> YTPVEEKENGRMIVIVPKKYEEDIEDFVDWKNQRGLRTEVKVAEDIASPVTANAIQQFVKQEYEKEGNDLTYVLLVGDHKDIPAKITPGIKSDQVYGQIVGNDHYNEVFIGRFSCESKEDLKTQIDRTIHYERNITTEDKWLGQALCIASAEGGPSADNGESDIQHENIIANLLTQYGYTKIIKCYDPGVTPKNIIDAFNGGISLANYTGHGSETAWGTSHFGTTHVKQLTNSNQLPFIFDVACVNGDFLYNVPCFAEALMRAQKDGKPTGTVAIIASTINQSWASPMRGQDEMNEILCEKHPNNIKRTFGGVTMNGMFAMVEKYKKDGEKMLDTWTVFGDPSLLVRTLVPTKMQVTAPANISASAQTFEVACDYNGAIATLSDDGDMVGTAIVKDGKAIIKLNESIADETNLTLTVVGYNKVTV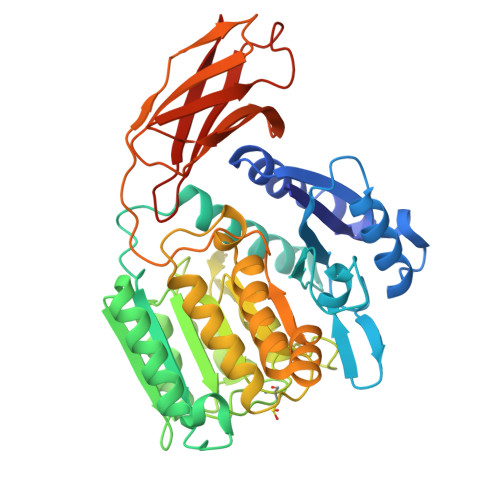IKDVKVEGHHHHHH>MNTAVEPYKASSFDDTHKLTVEKHGHTALITINHPPANTWDRDSLIGLRQLIEHLNRDDDIYALVVTGQGPKFFSAGADLNMFA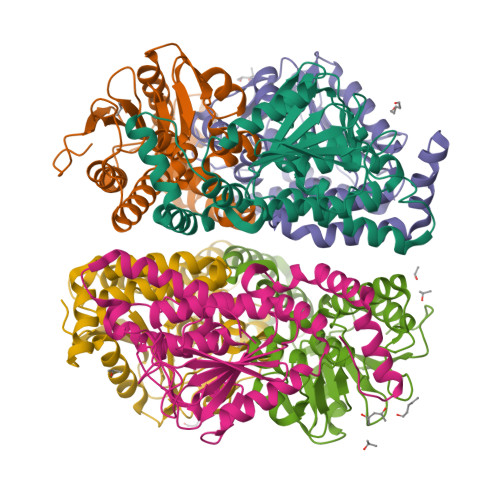DGDKARAREMARRFGEAFEALRDFRGVSIAAINGYAMGGGLECALACDIRIAERQAQMALPEAAVGLLPCAGGTQALPWLVGEGWAKRMILCNERVDAETALRIGLVEQVVDSGEARGAALLLAAKVARQSPVAIRTIKPLIQGARERAPNTWLPEERERFVDLFDAQDTREGVNAFLEKRDPKWRNCLEHHHHHH[6x]>[4x]MLDANKLQQAVDQAYTQFHSLNGGQNADYIPFLANVPGQLAAVAIVTCDGNVYSAGDSDYRFALESISKVCTLALALEDVGPQAV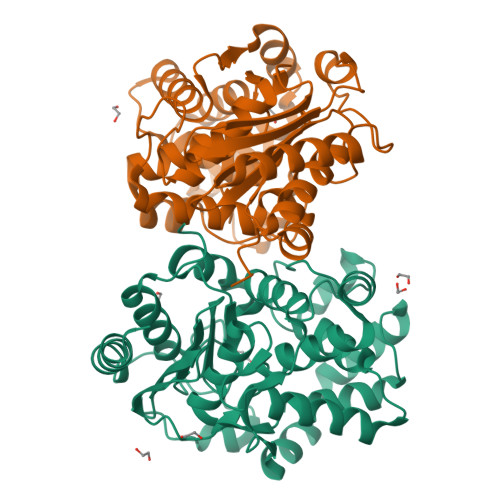QDKIGADPTGLPFNSVIALELHGGKPLSPLVNAGAIATTSLINAENVEQRWQRILHIQQQLAGEQVALSDEVNQSEQTTNFHNRAIAWLLYSAGYLYCDAMEACDVYTRQCSTLLNTIELATLGATLAAGGVNPLTHKRVLQADNVPYILAEMMMEGLYGRSGDWAYRVGLPGKSGVGGGILAVVPGVMGIAAFSPPLDEDGNSVRGQKMVASVAKQLGYNVFKG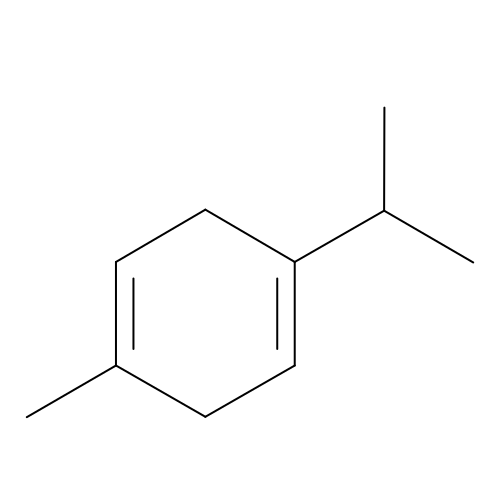1-methyl-4-(propan-2-yl)cyclohexa-1,4-diene | C10 H16 | YKFLAYDHMOASIY-UHFFFAOYSA-N>DVVRASRNAKVKGKFRESYLSPAQSVKPKINTEEKLPREKLNPPTPSIYLESKRDAFSPVLLQFCTDPRNPITVIRGLAGSLRLNLGLFSTKTLVEASGEHTVEVRTQVQQPSDENWDLTGTRQIWPCESSRSHTTIAKYAQYQASSFQESLQEEKESEDEESEEPDSTTGTPPSSAPDPKNHHIIKFGTNIDLSDAKRWKPQLQELLKLPAFMRVTSTGNMLSHVGHTILGM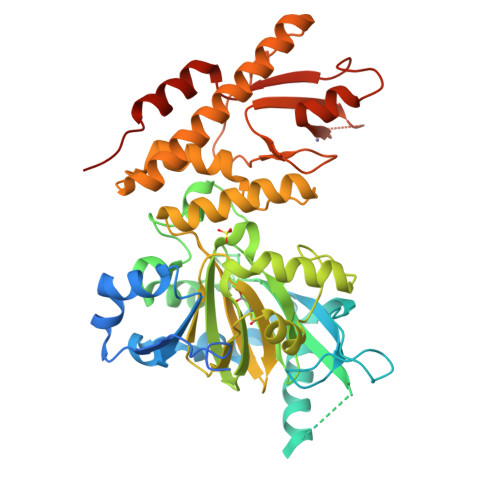NTVQLYMKVPGSRTPGHQENNNFCSVNINIGPGDCEWFAVHEHYWETISAFCDRHGVDYLTGSWWPILDDLYASNIPVYRFVQRPGDLVWINAGTVHWVQATGWCNNIAWNVGPLTAYQYQLALERYEWNEVKNVKSIVPMIHVSWNVARTVKISDPDLFKMIKFCLLQSMKHCQVQRESLVRAGKKIAYQGRVKDEPAYYCNECDVEVFNILFVTSENGSRNTYLVHCEGCARRRSAGLQGVVVLEQYRTEELAQAYDAFTLAPASTSRHHHHHH[2x]>[3x]AELCNKQQQQGPFTFANYQESPLNVSRLQIKVTKTTVQDRGKNFIIGYRAYWRSYCYNGGSLDGNTGCYNSLNPKPPTKDELKTWGQEEVCYTGPEVQDAWSGDSSICFVDWKMDNKHRAKELEKRSNNNHFAHHTCNLSWRCGVTNTHLEVRLVASGTQPQAVIVMPNGTTRAVSMVAETFWTDGEFSYLYSPKVFGTRAETKFIPCFKEHVKTRLDQGG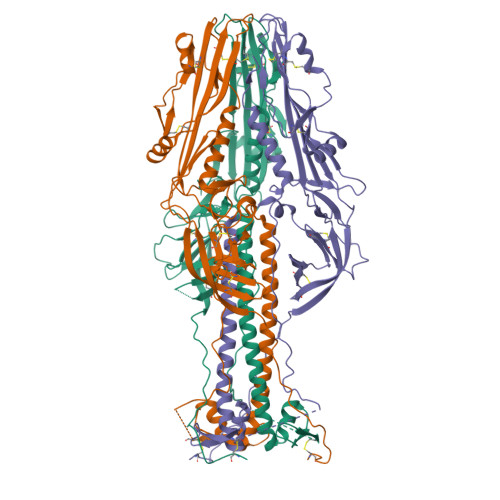SDYLIHDLTTEKFHCKDGDNFFEFPSSGFICLPDACYKNEKQKNNLLHPGMWNISEKLHAASVYDVNNVIHSLVYETESLRLSLAQLDHRFSVLTKLMNKMVSSLAKIDDRLIGALLEKPMASKFISPTKFMVSPCVAVLEEESNCHKDSIYRDGRWVYNNDPTKCFILNSSQTIDLFNFKTLWLPQLVAAKVEGVVSDEDGWTFVANSKQALLDTMTYTKNGGRGTSMEDVLNYPSGWLSGKLNG> MSETKPKYNYVNNKELLQAIIDWKTELANNKDPNKVVR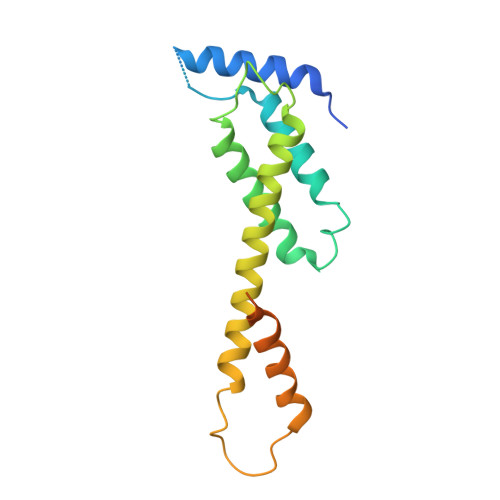QNDTIGLAIMLIAEGLSKRFNFSGYTQSWKQEMIADGIEASIKGLHNFDETKYKNPHAYITQACFNAFVQRIKKERKEVAKKYSYFVHNVYDSRDDDMVALVDETFIQDIYDKMTHYEESTYRTPGAEKKSVVDDSPSLDFLYEAND>[4x]HHHHHHFNLPPGNYKKPVLLKSTETGQYLRINPDGTVDGTRDRSDQHIQFQISPEGGGEVLLKSTETGQYLRINPDGTVDGTRDRSDQHIQFQISPEGGGEVL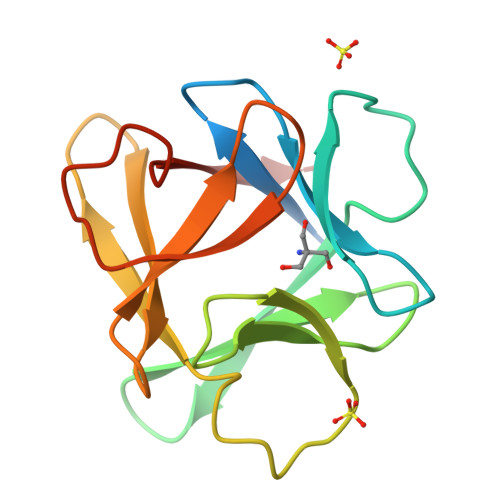LKSTETGQYLRINPDGTVDGTRDRSDQHIQFQISPEGGG uridine 5'-heptaphosphate | C9 H19 N2 O27 P7 | 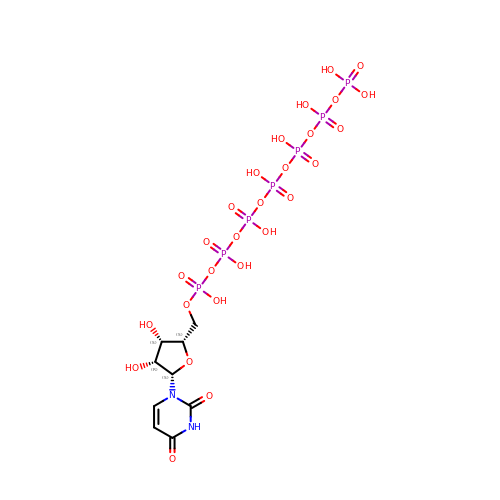DLYGIJYUJNEFKD-IHBLQFBFSA-N>YSHTATPAITLPSSGSANFAGVEYPLLPLDQHTPLLFQWFERNPSRFGENQIPIINTQQNPYLNNIINAAIIEKERTIGVLVDGNFSAGQKKALAKLEKQYENIKVIYNSDLDYSMYDKKLSDIYLENIAKIEAQPANVRDEYLLGEIKKSLNEVLKNNPEESLVSSHDKRLGHVRFDFYRNLFLLKGSNAFLEAGKHGCHHLQPGGGCIYLDADMLLTGKLGTLYLPDGIAVHVSRKGNSMSLENGIIAVNRSEHPALKKGLEIMHSKPYGDPYIDGVCGGLRHYFNCSIRH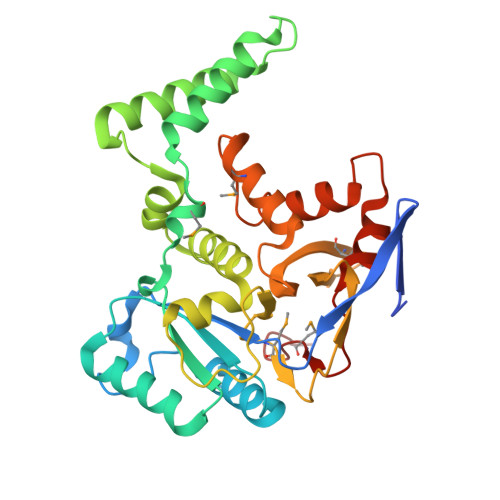NYEEFCNFIEFKHEHIFMDTSSLTISS[4x]The Endosomal Sorting Complexes Required for Transport (ESCRT) pathway drives multiple cellular membrane fission processes through the formation of filaments comprising different subsets of related ESCRT-III family members. ESCRT-III filaments stabilize highly curved membrane necks that resolve by fission when the filaments are remodeled by Vps4. Vps4 is monomeric or dimeric at cytoplasmic concentrations, but forms a hexamer when active and recruited to ESCRT-III filaments. The Vps4 N-terminal MIT domain is followed by an ~40 residue flexible linker and an ATPase cassette that comprises a large ATPase domain, small ATPase domain, and a β domain.

The new reconstruction of the Vps4-Vta1-ESCRT-IIIpeptide-ADP·BeFx complex agrees well with our earlier 4.3 Å resolution reconstruction but now has an overall resolution of 3.2 Å, which likely reflects the use of superior microscope instrumentation. The six Vps4 subunits form a closed ring, with six Vta1 VSL domains binding around the periphery and a single ESCRT-III peptide bound in the central pore (Figure 1—figure supplements 1–4). Subunit E deviates slightly from the more exact helical symmetry of subunits A-D. The large domain of subunit F is disengaged from adjacent Vps4 subunits (and substrate) and appears to be transitioning between the two ends of the Vps4 helix. Subunit F and features at the ring periphery, including the Vps4 β domains and the Vta1 VSL domains, have weak density. The density of subunit F is too weak to reliably assess the presence of nucleotide, and it may be empty. In contrast to the major disruption in contacts between the large domain of subunit F and the large domains of its neighbors, contacts involving the small ATPase domains remain more similar. This is especially true for the FA interface, where the F small domain to A large domain contacts are closely superimposable with those of AB, BC, CD, and DE. The E small domain to F large domain contacts are mediated by the same hydrophobic contacts, albeit with a rotation of ~25° and attendant shifts of 4.5–7.5 Å. Thus, this interaction appears to be maintained throughout the reaction cycle as subunits transition from the lagging (subunit E) to the leading (subunit A) end of the Vps4 helix, and may help maintain the hexameric assembly while the hydrolysis and release of ATP disrupts the core large domain contacts that define the ESCRT-III substrate-binding site. The specific point in the reaction cycle captured in our structure corresponds to subunit E just starting to transition toward the F state, as indicated by the slight deviation of the DE interface from the configuration of AB, BC, and CD, and consistent with our structural interpretation that ADP is bound to subunit D (above).

>[6x]GQEEGEDNGGEDNKKLRGALSSAILSEKPNVKWEDVAGLEGAKEALKEAVILPVKFPHLFKGNRKPTSGILLYGPPGTGKSYLAKAVATEANSTFFSVSSSDLVSKWMGESEKLVKQLFAMARENKPSIIFIDEVDALTGTRGEGESEASRRIKTELLVQMNGVGNDSQGVLVLGATNIPWQLDSAIRRRFERRIYIPLPDLAARTTMFEINVGDTPCVLTKEDYRTLGAMTEGYSGSDIAVVVKDALMQPIRKIQSATHFKDVSTEDDETRKLTPCSPGDDGAIEMSWTDIEADELKEPDLTIKDFLKAIKSTRPTVNEDDLLKQEQFTRDFGQEGNGGGGSGGGGSGGGGSGGGMAVDMFIKIGDVKGESKDKTHAEEIDVLAWSWGMSQSGSMHMGGGGGAGKVNVQDLSFTKYIDKSTPNLMMACSSGKHYPQAKLTIRKAGGENQVEYLIITLKEVLVSSVSTGGSGGEDRLTENVTLNFAQVQVDYQPQKADGAKDGGPVKYGWNIRQNVQAG;> XDEIVNKVLX;>[12x]MASNAARVVATAKDFDKVGLGIIGYYLQLYAVELILSEEDRSQEMTALATELLDTIEAFKKEIGGESEAEDSDKSLHVMNTLIHDQEKAKIYMLNFTMSLYNEKLKQLKDGPWDVMLKRSLWCCIDLFSCILHLWKENISETSTNSLQKRIKYCKIYLSKLAKGEIGSSDEKTLDYADFADDSEEIKDEDVDHQTSDLENNNNDKVEGLAPKDQTTSYEPVDEVPEFIDDADSVNEEEQTVDKNEDAITKDEQQVVKKEVDLTRPSAPSEPAAAEHKSYTKDELTKIMDRASKIEQIQKLAKYAISALNYEDLPTAKDELTKALDLLNSI>[2x]HHHHHHSSGLVPRGSHMASQVVRIVGVGRTGIGKLHKSVDELAASALKCALVDANMKQCDLQALIAVPSLASPQFMQAHHIATVAGLFPTKGKFIVRTVDTGGAGPITALGMAVDLVRTRCAETVAVIAADAVLSMGSGAFAERSNASLRRSGLPEPCIPHGYDRYAQWYMSRYGLKR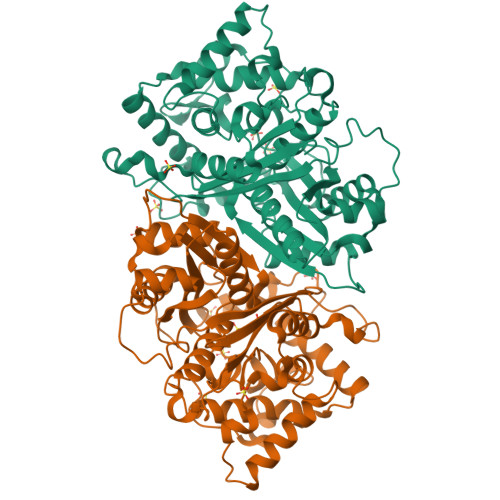EQLAMVPVLMSKMAERHPEAMCQKAYTLDEVLHSRCVAPVTNLLECARRADGAVALIVSGEAHYAEHFAQGKQEQRHLGGSKPIIASVAEASGPLFPPGSSDDIVPDIFSCRHAARDAFLSANLNVGDIHFFGLYDCFPICLIQAVEAVGLCPEGKGGEFMETAYNEMLNNGGVLDPSKFPINTHGGLQCFGAPWEVPAMYNITEAIAQLSEEAGDRQLTPVPKRALVYGNGGIFSASSVAILISDL1,4-BIS-[2-(2-HYDROXY-ETHYLAMINO)-ETHYLAMINO]-ANTHRAQUINONE | C14 H8 O2 | 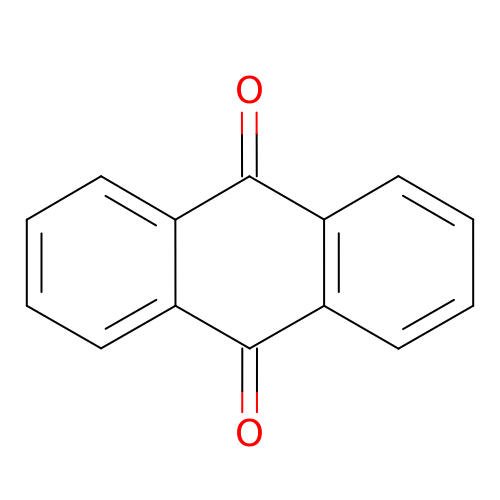RZVHIXYEVGDQDX-UHFFFAOYSA-N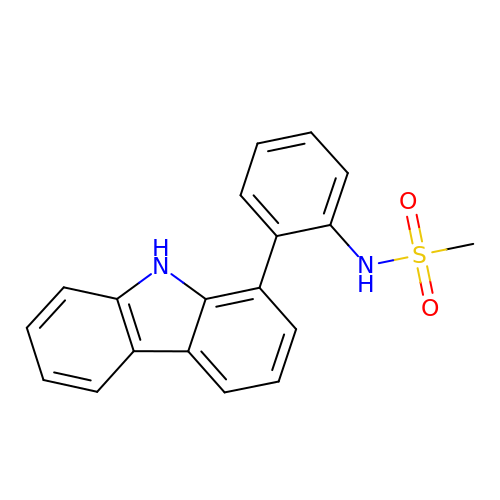~{N}-[2-(9~{H}-carbazol-1-yl)phenyl]methanesulfonamide | C19 H16 N2 O2 S | FKXDARRJLQDNOV-UHFFFAOYSA-N N'-{(1S,2R)-1-(3,5-DIFLUOROBENZYL)-2-HYDROXY-2-[(2R,4R)-4-PHENOXYPYRROLIDIN-2-YL]ETHYL}-5-METHYL-N,N-DIPROPYLISOPHTHALAMIDE 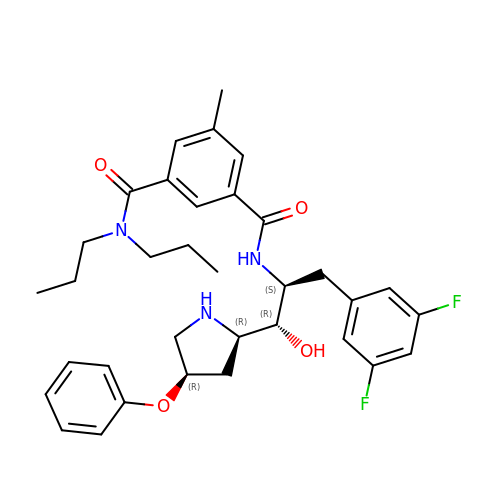| C34 H41 F2 N3 O4 | YDCNYSQITCUGST-FEFKUCBWSA-N>MASKKVCIVGSGNWGSAIAKIVGGNAAQLAQFDPRVTMWVFEEDIGGKKLTEIINTQHENVKYLPGHKLPPNVVAVPDVVQAAEDADILIFVVPHQFIGKICDQLKGHLKANPTGISLIKGVDEGPNGLKLI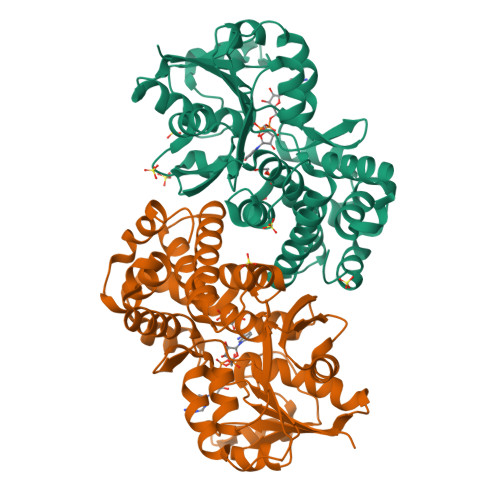SEVIGERLGIPMSVLMGANIASEVADEKFCETTIGCKDPAQGQLLKELMQTPNFRITVVQEVDTVEICGALKNVVAVGAGFCDGLGFGDNTKAAVIRLGLMEMIAFAKLFCSGPVSSATFLESCGVADLITTCYGGRNRKVAEAFARTGKSIEQLEKELLNGQKLQGPETARELYSILQHKGLVDKFPLFMAVYKVCYEGQPVGEFIHCLQNHPEHM[2x]>[2x]PISADFSEVENAPSFLSLAENTDEVLKPYTGLEIQTIITNIVGDANPNQSRIFDQDRLRGNQYSAGGLVTQNAVSAIPFTNLIPRTIRVGNILVNSANRLQITETNVSEYYSNPIIATKLSEMISDQVKNNQFSTWRRDNTSLQGFNAFDIATINTAILPNGLSLESMLLKLSLLHSIKAMNVDAASINRSQYQVIDHNTVPTIGAPAVVGVNNSPVFGEDCGGNNPVYPFGGGTGAIAFHVTLQTVPDERKSYAIFVPPAILQATSDANEALALFALSMSEWPHALYTVTKQTTDLAGANAGQQVFIPTQSTIHIGGRRVLDLIIPRREIAPNPTTLVAANAMCMVRPQAGPDATAGAIPLAAGQLFNMNFIGAPAFEEWPMTSYLYSWAGRFDITTIRQYMGRLATMVGVKDAYWAAHELNVALSQVAPKMTTAAGGWAAQAANSAQQSDVCYSSLLTVTRSAANFPLANQPAADMRVYDTDPATWNKVALGLATAANL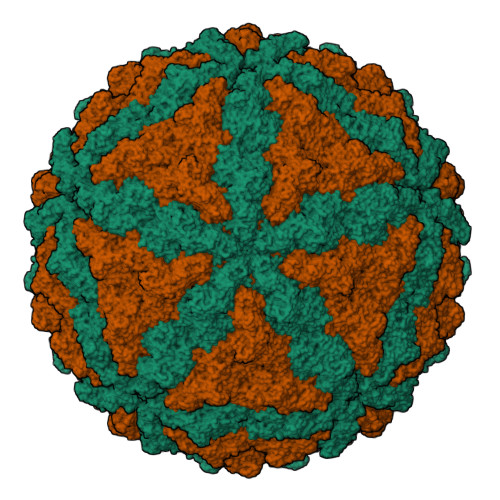VPEQSMDVPFVVGDARASFWERLQAIPMCIAWTMYYHSRGITTLAWDNAYTDNTNKWLQKMVRNTFSTTQSVGTIIPARYGKIVCNLYKNMFHRAPAYVATSVGGKELHITHFERWLPGGTYANVYSGAGAVVNCFSPVLIPDIWCQYFTAKLPLFAGAFPPAQGQNSTKGFNSKQGLMIHRNQNNNLVAPYLEKFADNSSYFPVGQGPEINDMATWNGRLWMTTGNVQYLDYSGAAIVEAVPPAGELPVGKQIPLLAGENAPIELTNAATTCVPRYSNDGRRIFTYLTTAQSVIPVQACNRAANLARSCWLLSNVYAEPALQALGDEVEDAFDTLTNSSFLDVAKSVAESAGEVPATKALTDLQAVDVSSLPSTSDPSNVLSQPAPLMSPPTSSS>[2x]HHHHHHGLIQERRSHEVNPAAHLTGANSSLTGSGGPLLWETQLGLAFLRGLSYHDGALVVTKAGYYYIYSKVQLGGVGCPLGLASTITHGLYKRTPRYPEELELLVSQQSPCGRATSSSRVWWDSSFLGGVVHLEAGEEVVVRVLDERLVRLRDGTRSYFGAFMV;>[2x]VAETPTYPWRDA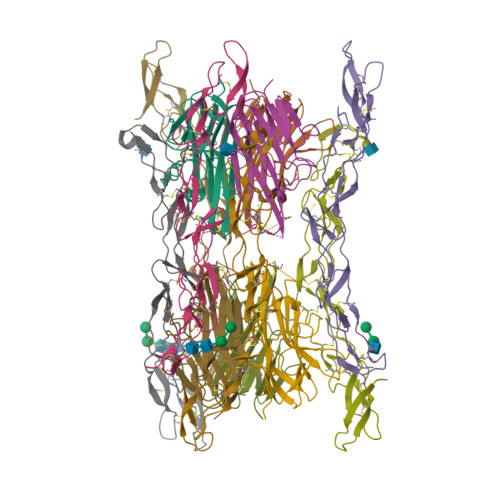ETGERLVCAQCPPGTFVQRPCRRDSPTTCGPCPPRHYTQFWNYLERCRYCNVLCGEREEEARACHATHNRACRCRTGFFAHAGFCLEHASCPPGAGVIAPGTPSQNTQCQPCPPGTFSASSSSSEQCQPHRNCTALGLALNVPGSSSHDTLCTSTGHHHHHH4'-chloro-N-[(1R)-2-(1H-imidazol-1-yl)-1-phenylethyl]biphenyl-4-carboxamide 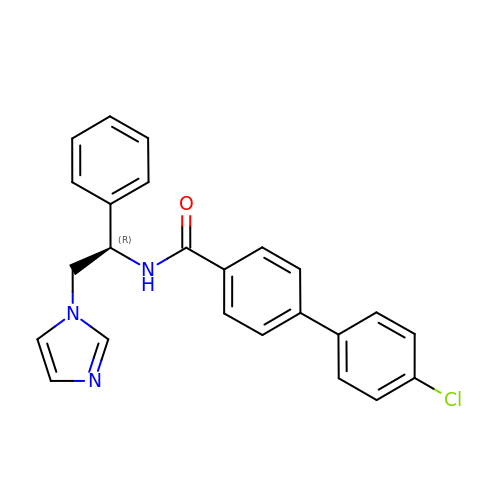| C24 H20 Cl N3 O | CIFIVCCKVZFJFT-QHCPKHFHSA-N>MGEIESYCNKELGPLPTKAPTLSKNVLDLFSLKGKVASVTGSSGGIGWAVAEAYAQAGADVAIWYNSHPADEKAEHLQKTYGVHSKAYKCNISDPKSVEETISQQEKDFGTIDVFVANAGVTWTQGPEIDVDNYDSWNKIISVDLNGVYYCSHNIGKIFKKNGKGSLIITSSISGKIVNIPQLQAPYNTAKAACTHLAKSLAIEWAPFARVNTISPGYIDTDITDFASKDMKAKWWQLTPLGREGLTQELVGGYLYLASNAS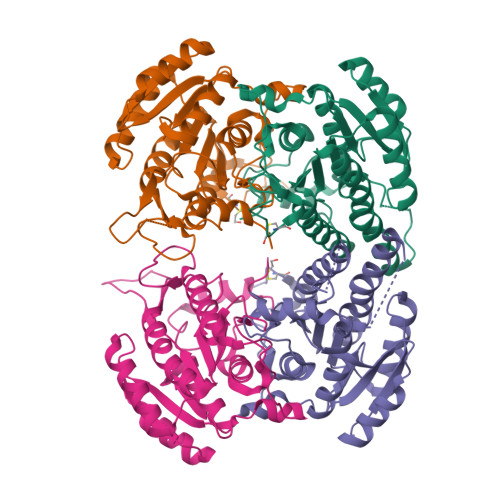TFTTGSDVVIDGGYTCPLEHHHHHH[8x]5-CHLORO-1H-INDOLE-2-CARBOXYLIC 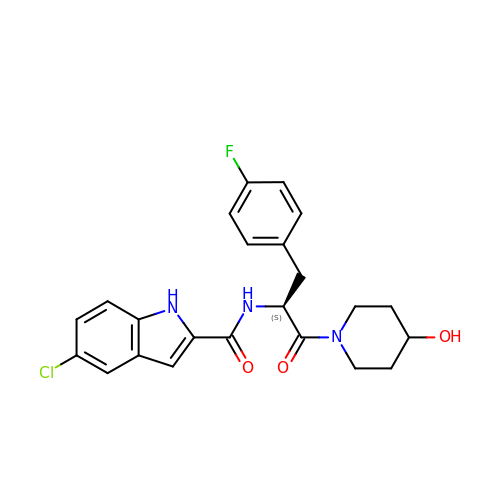ACID [1-(4-FLUOROBENZYL)-2-(4-HYDROXYPIPERIDIN-1YL)-2-OXOETHYL]AMIDE | C23 H23 Cl F N3 O3 | YDCGVASFVACWKF-NRFANRHFSA-N>[2x]MGNKNTPLNSGKHPDLKIEVAIIGAGTSGLYTAYRLVTDKKFKAHDVQIFDMNNKLGGRLESVIMPGMNFWGELGGMRYLTSQQIVTTLIEGYPLSEKDPNKRTPVLKDKMTPVPFPMGDPSKLLMYLRKERFKQNAWNEAQKKGEKLPTRYYLNENDLGFSSDQLFNKIIYDVLMADPWVAETYGSKIIKGSSVYDYSFKLTSRDWDDIKPKLVYNFPNSPYDQRKVNDIGFWNLIKDQVSQEGYEFLANAGGYYSNTINWNSAEAFPYMVGDFSAGTIYKTIEEGYDSIAYAVANSYMEHEGACIWSENKLLTFTKDHPLTNTHKYELTFLNLKTNTQWKVYANSIVLAMPRKSLELLDQNNFFFNINKNSVLNNNIRSVIMEPAFAILMGFEYPWWKELGIDSGHSITDLPMRQCYYFGTDPETNNSMLLGSYGDMETETFWKALSDDKVLFEVKAAKSASLRELHQLDDVQATKLMVGELMNQLRELHGDTVTIPEPYVTYFKDWTDEPFGAGYHAWKAGFSVENVMPYMRKPLTDEQIHICGEAYSDQQGWVEGAFCEAEKMLQEYFGLDRPYWLSPDYYLGWEHHHHHH

Progenitor sequence of the assigned 28 sequences was generated by ancestral sequence reconstruction, and the generated sequence exhibited L-lysine oxidase activity; thus, we named the enzyme AncLLysO. AncLLysO has a fold typical of the flavin-dependent amine oxidase (FAO) superfamily —the Rossmann-core fold, which recognizes FAD, and a hot-dog-like fold, which is important for the recognition of substrates. Taken together, we assigned a novel FAD-dependent enzyme, called LLysO and bearing a main L-Lys α-oxidase and promiscuous monooxygenase activity, from the database. The main-chain amino group of L-Lys is deprotonated by an activated solvent water molecule, and the hydride on the main-chain carbon atom is transferred to FAD.

Previous research indicates that, in many FAD-dependent oxidases, the Lys residue at the site would recognize the O2 molecule, which oxidizes the FADH2, and their variants quietly reduce the activity. In AncLLysO, K387 corresponds with the residue, and the activity of the AncLLysO(K387A) variant was reduced below the detection limit of the activity assay as expected. Crystal structures of the L-Lys- and L-Arg-binding forms of AncLLysO(K387A) were determined at 2.4- and 2.2-Å resolution, respectively, using the cocrystallization method. In general, fitting of substrates into an electron density map would be difficult at the resolution of the AncLLysO(K387A) structure; however, the substrates appeared to be fitted into the map appropriately. In fact, the polder Fo-Fc omit map indicates that L-Lys and L-Arg coordinate at the active site using different binding modalities; a stereo view of L-Lys- and L-Arg-binding forms is shown in Fig. S3. Differences in the binding mode would affect the substrate specificity of AncLLysO. In fact, the main-chain carbon atom of L-Arg is moved to the arrowed direction approximately 1.5 Å compared with L-Lys. Because of this movement, the distance between the main-chain carbon atom of L-Arg and the N5 atom of FAD is about 1.2 Å longer than in the case of L-Lys. This causes inefficient hydride transfer of Cα-H from L-Arg to the N5 atom of FAD during the reaction by AncLLysO. From a structural comparison between the ligand-free form and the L-Lys- or L-Arg-binding form of AncLLysO, substrate binding appeared to induce a conformational change of a loop that is formed by residues 251 to 254 (251-GGYY-254); cis–trans transformation at G251 is remarkable in this change.> MGSDKIHHHHHHMETQDYAFQPGLTVGELLKSSQKDWQAAINHRFVKELFAGTIENKVLKDYLIQDYHFFDAFLSMLGACVAHADKLESKLRFAKQLGFLEADEDGYFQKAFKELKVAENDYLEVTLHPVTKAFQDLMYSAVASSDYAHLLVMLVIAEGLYLDWGSKDLALPEVYIHSEWINLHRGP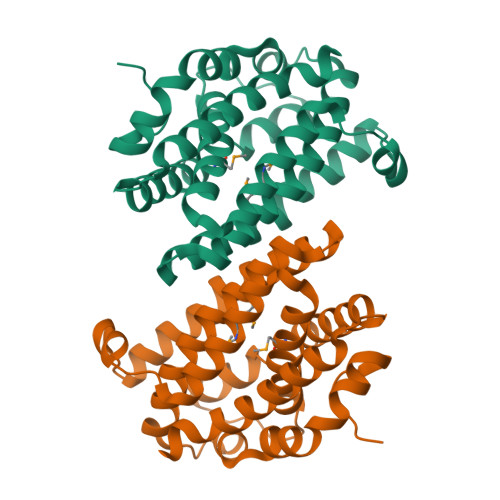FFAEWVQFLVDELNRVGKNREDLTELQQRWNQAVALELAFFDIGYDV> MIDLDFRKLTIEECLKLSE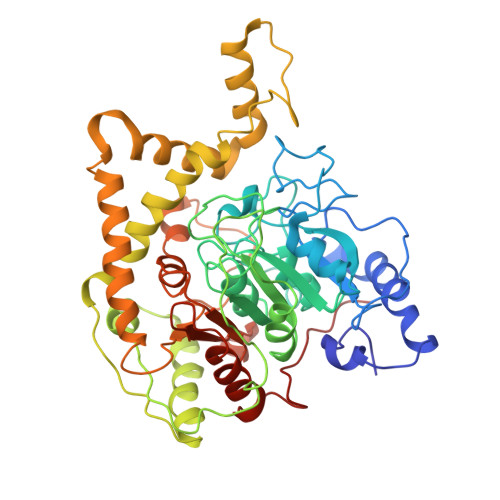EEREKLPQLSLETIKRLDPHVKAFISVRENVSVEKKGKFWGIPVAIKDNILTLGMRTTCASRILENYESVFDATVVKKMKEAGFVVVGKANLDEFAMGSSTERSAFFPTRNPWDLERVPGGSSGGSAAAVSAGMVVAALGSDTGGSVRQPASLCGVVGYKPTYGLVSRYGLVAFASSLDQIGPITKTVRDAAILMEIISGRDENDATTVNRKVDFLSEIEEGVSGMKFAVPEEIYEHDIEEGVSERFEEALKLLERLGAKVERVKIPHIKYSVATYYVIAPAEASSNLARFDGVKYGLRIKEKGLREMYMKTRNVGFGEEVRRRIMIGTFTLSAAYYEAYFNKAMKVRRKISDELNEVLSQYDAILTPTSPVTAFKIGEIKDPLTYYLMDIFTIPANLAGLPAISVPFGFSNNLPVGVQVIGRRFADGKVFRIARAIEKNSPYNENGMFPLPEVKA>[2x]EL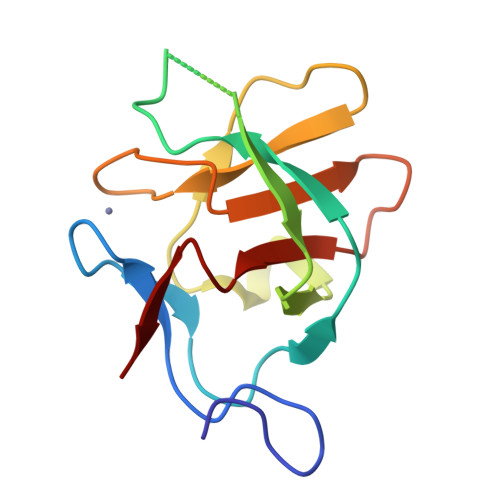VSAEGRNRKAVLCQRCGSRVLQPGTALFSRRQLFLPSMRKKPDLVDGSNPDGDVLEEHWLVNDMFIFENVGFTKDVGNVKFLVCADCEIGPIGWHCLDDKNSFYVALERVSHE>[2x]MATAQSNSPRVFCIGTADTKFDELRFLSEHVRSSLNSFSNKSSFKVGVTVVDVSTSWKETNSCADFDFVPSKDVLSCHTLGEETMGTFADIRGLAIAIMSKALETFLSIANDEQNLAGVIGLGGSGGTSLLSSAFRSLPIGIPKVIISTVASGQTESYIGTSDLVLFPSVVDICGINNVSKVVLSNAGAAFAGMVIGRLESSKEHSITNGKFTVGVTMFGVTTPCVNAVKERLVKEGYETLVFHATGVGGRAMEDLVRGGFIQGVLDITTTEVADYVVGGVMACDSSRFDAILEKKIPLVLSVGALDMVNFGPKTTIPPEFQQRKIHEHNEQVSLMRTTVGENKKFAAFIAEKLNKASSSVCVCLPEKGVSALDAPGKDFYDPEATSCLTRELQMLLENNERCQVKVLPYHINDAEFANALVDSFLEISPK;>[2x]SYTRSEEIESLEQFHMATASSLIHKQMCSIVYTGPLKVQQMKNFIDSLVASLSAAV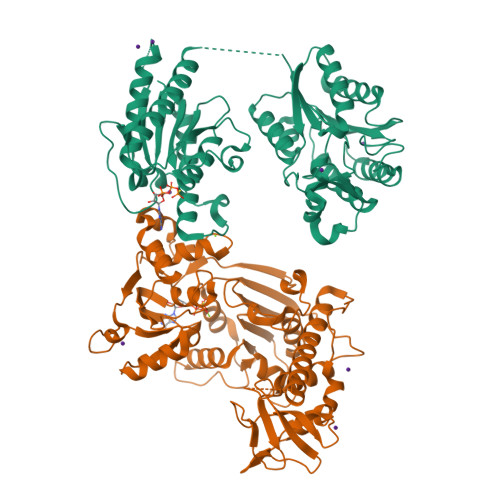SNLVKILKDTAAIDLETRQKFGVLDVASKRWLVKPSAKNHAWGVVETHARKYHVALLEHDEFGIITCDNWRRVAVSSESVVYSDMAKLRTLRRLLKDGEPHVSSAKVVLVDGVPGCGKTKEILSRVNFEEDLILVPGRQAAEMIRRRANASGIIVATKDNVRTVDSFLMNYGKGARCQFKRLFIDEGLMLHTGCVNFLVEMSLCDIAYVYGDTQQIPYINRVTGFPYPAHFAKLEVDEVETRRTTLRCPADVTHFLNQRYEGHVMCTSSEKKSVSQEMVSGAASINPVSKPLKGKILTFTQSDKEALLSRGYADVHTVHEVQGETYADVSLVRLTPTPVSIIARDSPHVLVSLSRHTKSLKYYTVVMDPLVSIIRDLERVSSYLLDMYKVDAGTQ>[3x]MGLRGKSGSTASSSLEGGSEFSERIGNSLSSFLSESASLEVIGNELADNIANEIVSSLQKDSASFLQSGFDVKTQLKATAKKVLVEALKAALEPTEKIVASTIKPPRVSED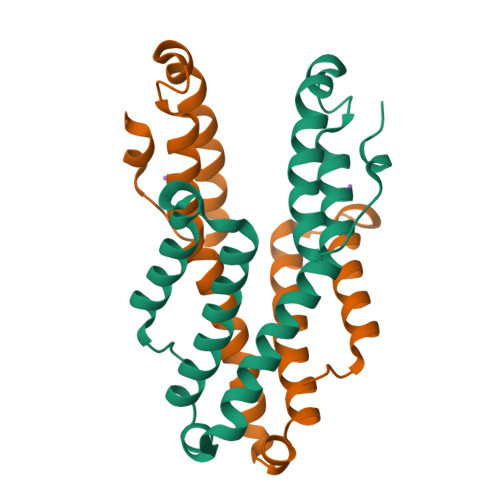AYFLLGPVVKTLFNKVEDVLHKPIPDTIWEYESKGSLEEEEAEDEFSDELLDLEHHHHHH> DRRHVLLQAEFYQRSEGPDKAWAQFGFHFDADELFHVELDAAQTVWRLPEFGRFASFEAQGALQNMAVGKQNLEVMISNSNRSQQDFVTPELALFPAEAVSLEEPNVLICYADKFWPPVATMEWRRNGAVVSEGVYDSVYYGRPDLLFRKFSYLPFVPQRGDVYSCAVRHWGA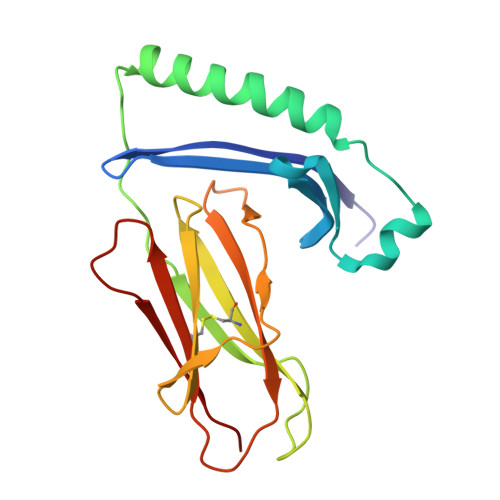EGPVQRMWEPE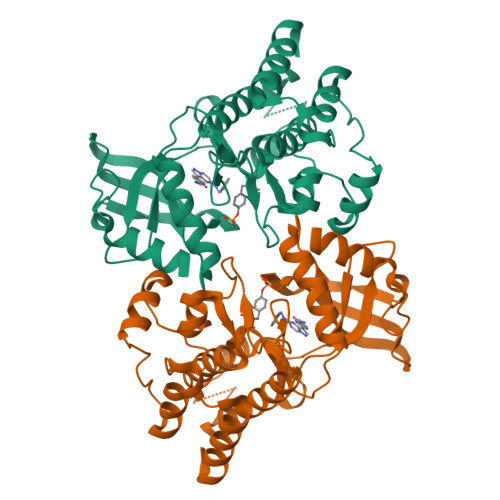> GPLSLSVDAFKILEDPKWEFPRKNLVLGKTLGEGEFGKVVKATAFHLKGRAGYTTVAVKMLKENASPSELRDLLSEFNVLKQVNHPHVIKLYGACSQDGPLLLIMEYAKYGSLRGFLRESRKVGPGYLGSGGSRNSSSLDHPDERALTMGDLISFAWQISQGMQYLAEMKLVHRDLAARNILVAEGRKMKISDFGLSRDVYEEDSYVKRSQGRIPVKWMAIESLFDHIYTTQSDVWSFGVLLWEIVTLGGNPYPGIPPERLFNLLKTGHRMERPDNCSEEMYRLMLQCWKQEPDKRPVFADISKDLEKMMVKRR>[2x]GSHMYLSKQLCFLFYVSS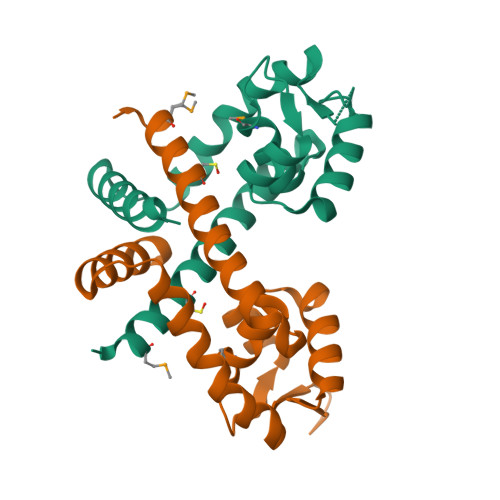KEIIKKYTNYLKEYDLTYTGYIVLMAIENDEKLNIKKLGERVFLDSGTLTPLLKKLEKKDYVVRTREEKDERNLQISLTEQGKAIKSPLAEISVKVFNEFNISEREASDIINNLRNFVSKNF> MSTYEGRWKTVKVEIEDGIAFVILNRPEKRNAMSPTLNREMIDVLETLEQDPAAGVLVLTGAGEAWTAGMDLKEYFREVDAGPEILQEKIRREASQWQWKLLRM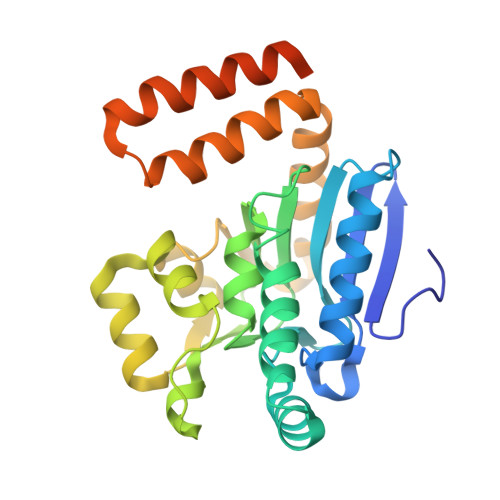YAKPTIAMVNGWCFGGGFSPLVACDLAICADEATFGLSEINWGIPPGNLVSKAMADTVGHRQSLYYIMTGKTFGGQKAAEMGLVNESVPLAQLREVTIELARNLLEKNPVVLRAAKHGFKRCRELTWQQNEDYLYAKLDQSRLLDTEGGREQGMKQFLDDKSIKPGLQAYKR(2S)-2-(dimethylamino)-4-(methylselanyl)butanoic acid | C7 H15 N O2 Se | 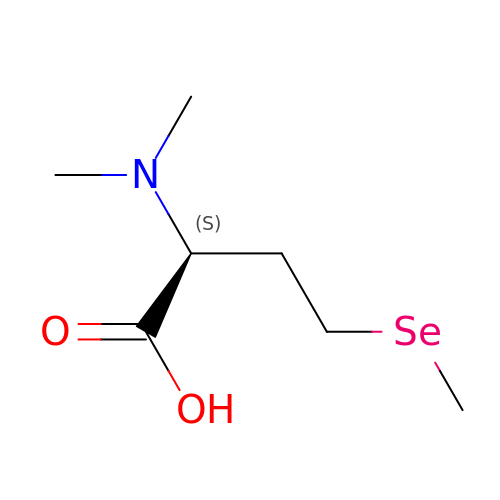HLLONANTKRYYCG-LURJTMIESA-N>[4x]MGSSHHHHHHSSENLYFQGGLVPRGSHMLSFDSNKEFALTRDLGVLKGIYLAPYMQVATALIGKARHAGGNMFRHQVDTMAILIDYGYIDSVLLKASLIHDVIENIE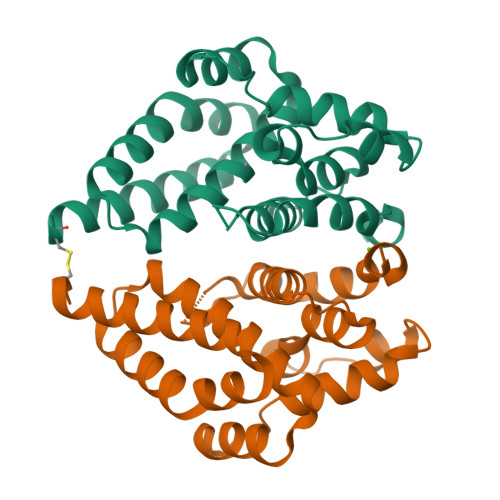DFNVNEILSIDSESGQVYELVLEVTKKKGQEKTEYLKNIIKNGSEKAKILKCADRISNMISLGFVTDSEFIERYCNETELYIFPIALEVNFEMYKELMALVVSRRQYLVECGYLEERVKKMRKAR> VSHQQGQSHLFECDYPISADTYVINWYKDGTSVMNYL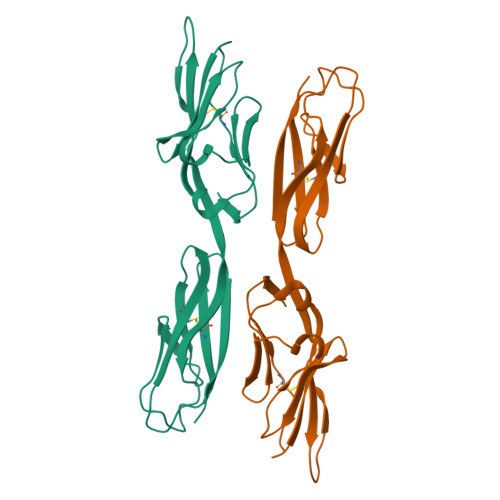SGGEPAFTEDLDDRTDVQFVNNRNLEITNLRVSDEGEYYCSVIEIGAGGQSGDGTRYQLVVFVPPTITLMGGPYEVEVGEMMMSTCRANSHPPSNFTWTLPNGNVTQGAVLEITNMTQAEIGTYMCTADNGYGTDYESVDITM> MSEEFIAVSTLARNLEIAKGNEFHTILATLRSPVYINEQLLKSELSFLVTKILKLIRSGNDFDLWKGCHTSVVTCAYNPLVLSTHGGQLLAAIYSRLEQKTGFYSSVISSSHGKQLFNTLISSVAIIIDLMKNKPTLSREALVPKLKAIIPTLITLSQYEPELVLPVLQRILKRNTTTFKPFTNKFRTVLINLIISDYASLGTKTQRLVCENFAYLHLLKIQVSDTSDDETQAHHKIYADSNWRTGLMSILSQFKPIIQLCGEILDFEQDNELYKLIKSLPVIDESNNKEEFLPSLKLDFNAPLTLWEIPQRLSLLADMLVAFISLPTPFPIRVPLGGINSLCEVLLGVSNKYLPLKKELRHDNELNGVINTILPQIQFQGIRLWEIMVSKYGKCGLSFFEGILSSIELFIPLKKKSNNEIDFNVVGSLKFEFATVFRLVNMILSHLGHQLNIISVISQLIEVALFLSHDKTLIDSLFKNRKSIMKQQTKTKQSKRSKSAEGAFSDIYTHPELFVCKNSMNWFNEINDFFITALNNWILPSTPHIQILKYSITQSLRLKERFGYIPESFVNLLRCEVLHPGSERVSILPIAISLLKNINDDMFELLCHPKVPVGMVYQLHKPLDLGEDGEVRDDINKKEVETNESSSNANTGLETLKALENLENVTIPEPKHEVPKVVDDTAIFKKRSVEEVIERESTSS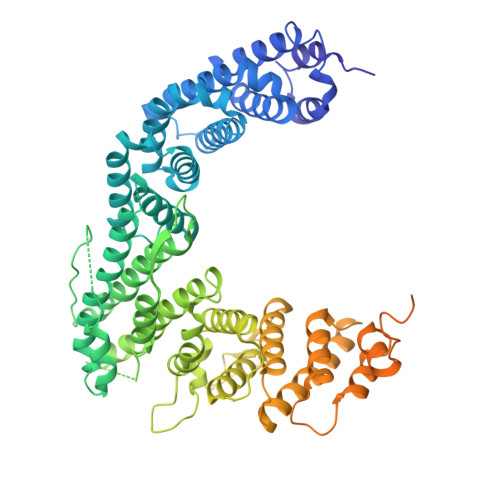HKKVKFVEETTVDNGEELIVKKAVSQTKEEEKPMEDSEDEEQEEFEIPAIELSDDEEEEEEEE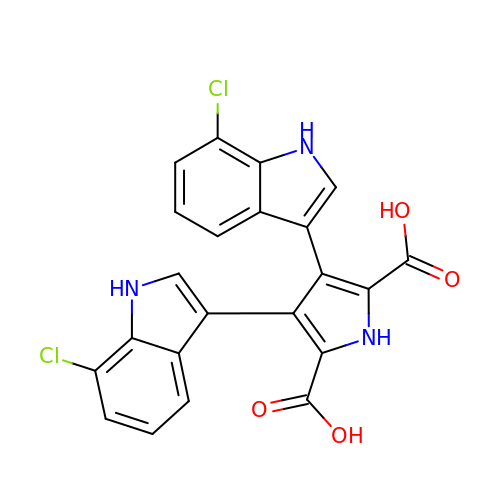3,4-bis(7-chloro-1H-indol-3-yl)-1H-pyrrole-2,5-dicarboxylic acid | C22 H13 Cl2 N3 O4 | OAMCCJASDLMTOO-UHFFFAOYSA-N>MARIRDVQGDITEFQGDAIVNAANNYLKLGAGVAGAILRKGGPSIQEECDRIGKIRVGEAAVTGAGNLPVRYVIHAAVLGDEPASLETVRKATKSALEKAVELGLKTVAFTVGGAWVGGLPAEAVCRVMREEIKKAPDTLEVTGVHGTEKSAEAPRRARL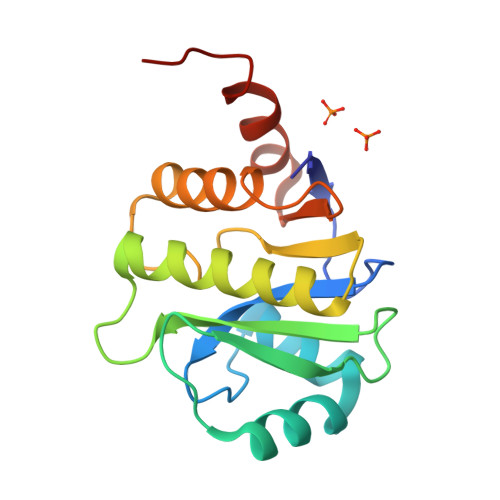EHHHHHH[2x]> MKKEVRKVRIALASPEKIRSWSYGEVEKPETINYRTLKPERDGLFDERIFGPIKDYECACGKYKRQRFEGKVCERCGVEVTRSIVRRYRMGHIELATPAAHIWFVKDVPSKIGTLLDLSATELEQVLYFNKYIVLDPKGAVLDGVPVEKRQLLTDEEYRELRYGKQETYPLPAGVDALVKDGEEVVKGQELAPGVVSRMDGVALYRFPRRVRVDYLRKERAALRIPLSAWVEKEAYRPGEVLAELSEPYLFRAEESGVVELKDLAEGHLIYLRQEEEVVARYFLPAGMTPLVVEGEIVEVGQPLAEGKGLLRLPRHMTAKEVEAEEEGDSVHLTLFLEWTEPKDYKVAPHMNVIVPEGAKVQAGEKIVAAIDPEEEVIAEAEGVVHLHEPASILVVKARVYPFEDDVEVTTGDRVAPGDVLADGGKVKSEIYGRVEVDLVRNVVRVVESYDIDARMGAEAIQELLKELDLEKLERELLEEMKHPSRARRAKARKRLEVVRAFLDSGNRPEWMILEAVPVLPPDLRPMVQVDGGRFATSDLNDLYRRLINRNNRLKKLLAQGAPEIIIRNEKRMLQEAVDAVIDNGRRGSPVTNPGSERPLRSLTDILSGKQGRFRQNLLGKRVDYSGRSVIVVGPQLKLHQCGLPKRMALELFKPFLLKKMEEKAFAPNVKAARRMLERQRDIKDEV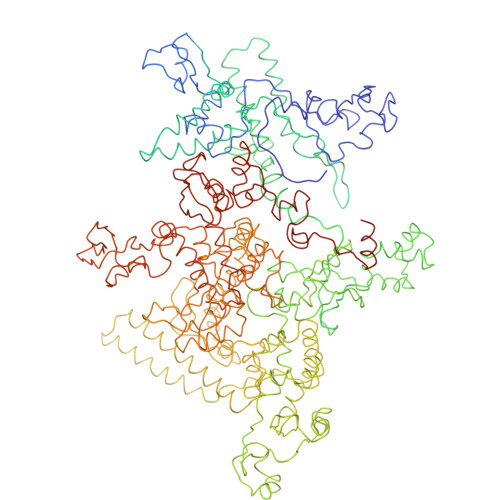WDALEEVIHGKVVLLNRAPTLHRLGIQAFQPVLVEGQSIQLHPLVCEAFNADFDGDQMAVHVPLSSFAQAEARIQMLSAHNLLSPASGEPLAKPSRDIILGLYYITQVRKEKKGAGMAFATPEEALAAYERGEVALNAPIVVAGRETSVGRLKFVFANPDEALLAVAHGLLDLQDVVTVRYLGRRLETSPGRILFARIVGEAVGDEKVAQELIQMDVPQEKNSLKDLVYQAFLRLGMEKTARLLDALKYYGFTLSTTSGITIGIDDAVIPEEKQRYLEEADRKLRQIEQAYEMGFLTDRERYDQVIQLWTETTEKVTQAVFKNFEENYPFNPLYVMAQSGARGNPQQIRQLCGMRGLMQKPSGETFEVPVRSSFREGLTVLEYFISSHGARKGGADTALRTADSGYLTRKLVDVAHEIVVREADCGTTNYISVPLFQMDEVTRTLRLRKRSDIESGLYGRVLAREVEALGRRLEEGRYLSLEDVHFLIKAAEAGEVREVPVRSPLTCQTRYGVCQKCYGYDLSMARPVSIGEAVGVVAAESIGEPGTQLTMRTFHTGGVAVGTDITQGLPRVIELFEARRPKAKAVISEIDGVVRIEEGEDRLSVFVESEGFSKEYKLPKDARLLVKDGDYVEAGQPLTRGAIDPHQLLEAKGPEAVERYLVDEIQKVYRAQGVKLHDKHIEIVVRQMLKYVEVTDPGDSRLLEGQVLEKWDVEALNERLIAEGKVPVAWKPLLMGVTKSALSTKSWLSAASFQNTTHVLTEAAIAGKKDELIGLKENVILGRLIPAGTGSDFVRFTQVVDQRTLKAIEEARKEAVEAKEKEAPRRPVRREQPGKGL> MHHHHMITLENPDIKYPL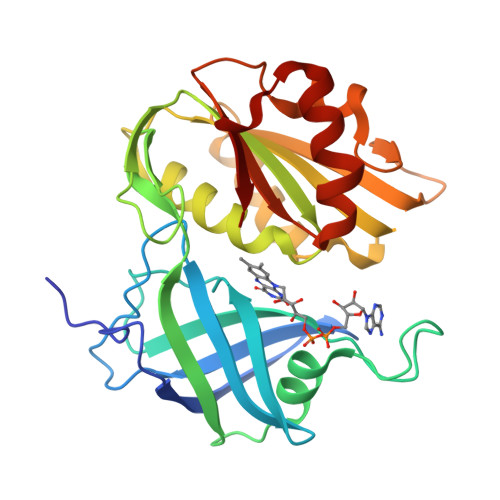RLIDKEILSHDTRRFRFALPSPQHILGLPIGQHIYLSTRIDGNLVIRPYTPVSSDDDKGFVDLVVKVYFKETHPKFPAGGKMSQYLENMNIGDTIEFRGPNGLLVYQGKGKFAIRADKKSNPVVRTVKSVGMIAGGTGITPMLQVIRAVLKDPNDHTVCYLLFANQSEKDILLRPELEELRNEHSSRFKLWYTVDKAPDAWDYSQGFVNEEMIRDHLPPPGEETLILMCGPPPMIQFACLPNLERVGHPKERCFTF> MPIGHSREVLVRLRDILALLADGCKTTSLIQQRLGLSHGRAKALIYVLEK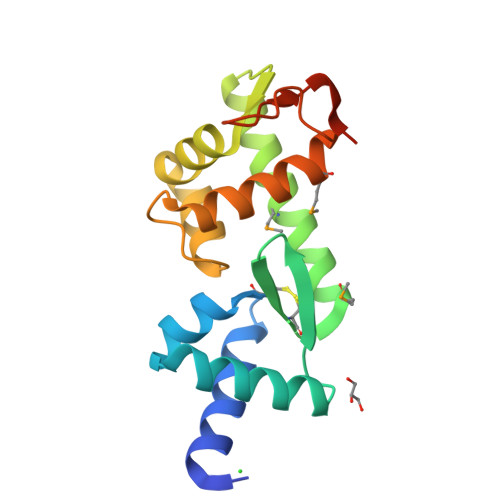EGRVTRVAFGNVALVCLSMDQYRQLVDGMIREVERLVTTNKLKFISPPRLHDLIIKDPQARKFFSSIIPIAHRTAIILSFLNHLLKMIYGEPYVKTDETVYLTANRKVHIEPPAK>HHHHHHLESTSLYKKAGSTPPRGVTVVNNFDAKRYLGTWYEIARFDHRFERGLEKVTATYSLRDDGGLNVINKGYNPDRGMWQQSEGKAYFTGAPTRAALKVSFFGPFYG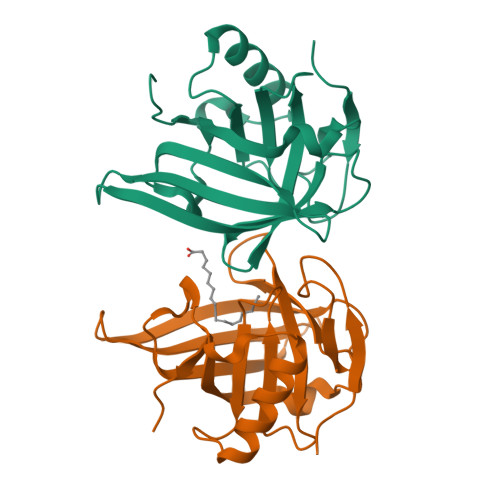GYNVIALDREYRHALVCGPDRDYLWILSRTPTISDEVKQEMLAVATREGFDVSKFIWVQQPGS[2x]>MGVVKGLLALALVLNVVVVSNGGKSSNFVRKTNKNRDMPLDSDVFRVPPGYNAPQQVHITQGDLVGRAMIISWVTMDEPGSSAVRYWSEKNGRKRIAKGKMSTYRFFNYSSGF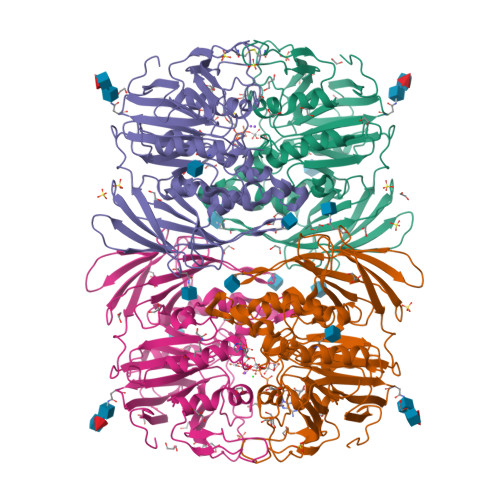IHHTTIRKLKYNTKYYYEVGLRNTTRRFSFITPPQTGLDVPYTFGLIGDLGQSFDSNTTLSHYELSPKKGQTVLFVGDLSYADRYPNHDNVRWDTWGRFTERSVAYQPWIWTAGNHEIEFAPEINETEPFKPFSYRYHVPYEASQSTSPFWYSIKRASAHIIVLSSYSAYGRGTPQYTWLKKELRKVKRSETPWLIVLMHSPLYNSYNHHFMEGEAMRTKFEAWFVKYKVDVVFAGHVHAYERSERVSNIAYKITNGLCTPVKDQSAPVYITIGDAGNYGVIDSNMIQPQPEYSAFREASFGHGMFDIKNRTHAHFSWNRNQDGVAVEADSVWFFNRHWYPVDDST[4x]> MATYKTPGVYIEEITKFPPSVAQVETAIPAFIGYTQFARTKPSVDSDDLILKPKRISSLLDFTTYYGGAQNEQGITVKLTDTLIEGAENRTINVPEPTFKSPYLMFYSLQMYFANGGGPCYIVSTGVYDDWSDSETPPTINFSDLESGLAVIRKEDEPTLLLFPDATNLPTDDEFYSLYNSALMQCNDLQDRFTILDTYSDQTYNDGVEDLDPIPALRNGINLTKDYLKYGAAYYPFVQTILNYQYSADEIVIQHLSYNPNAIATALDNLNAVNGPTFIDAILDDLRDLSLPDISGEISDAVGFMYDDVDGFDIDGTFTTNSVKVANFASLVESVLSTLNELIDAKEEINKDVNSAIASSEEDNAIKTAISDALDVFNEDFEGADKIESVAKNLSDLLIKIKQADTNTKVENVLSINALNFSAEFEKLLTYDVNTGLTASVTLDLFANIGTRLDDIIAAVSAAEPIDVNNGKLNGRLLSDIEPLDNATYNTILLEINSHKVTLPPSSSMAGAYARVDNDRGVWKSPANIGLNYVSKPSVTVSHEEQESMNVHGTGKSVNAIRSFVGKGTLVWGARTLAGNDNEWRYISVRRFFNMAEESIKKATEQFVFEPNDGNTWVRVRAMIENFLILQWRAGALAGAKPEHAFYVKVGLGQTMTAQDILEGNMNVEIGLAVVRPAEFIILKFSHKM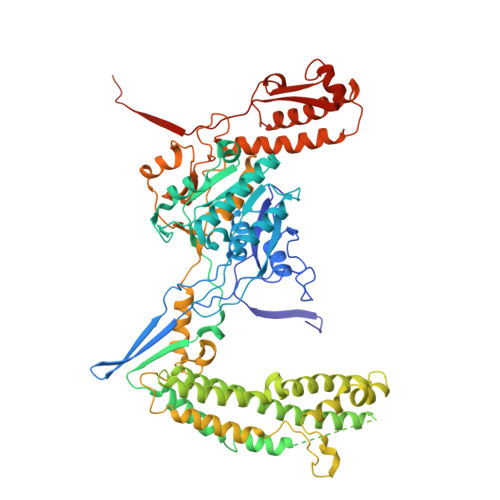QES>GSHMASMTGGQQMGRGSAAQRQGALAIMSRVYVGSIYYELGEDTIRQAFAPFGPIKSIDMSWDSVTMKHKGFAFVEYEVPEAAQLALEQMNSVM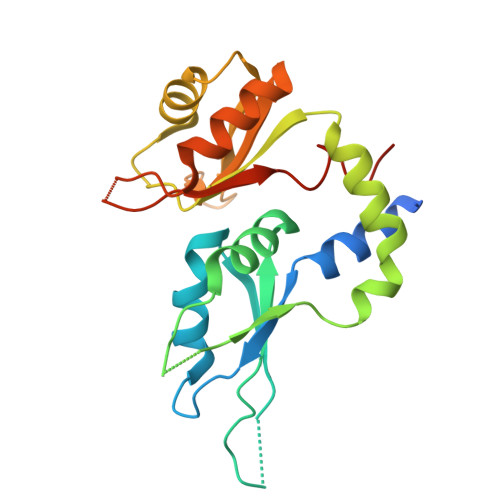LGGRNIKVGRPSNIGQAQPIIDQLAEEARAFNRIYVASVHQDLSDDDIKSVFEAFGKIKSATLARDPTTGKHKGYGFIEYEKAQSSQDAVSSMNLFDLGGQYLRVGKAVTPPMPLLTPATPG[2x]>MFKHTRKLQYNAKPDRSDPIMARRLQESLGGQWGETTGMMSYLSQGWASTGAEKYKDLLLDTGTEEMAHVEMISTMIGYLLEDAPFGPEDLKRDPSLATTMAGMDPEHSLVHGLNASLNNPNGAAWNAGYVTSSGNLVADMRFNVVRESEARLQVSRLYSMTEDEGVRDMLKFLLARETQHQLQFMKAQEELEEKYGIIVPGDMKEIEHSEFSHVLMNFSDGDGSKAFEGQVAKDGEKFTYQENPEAMGGI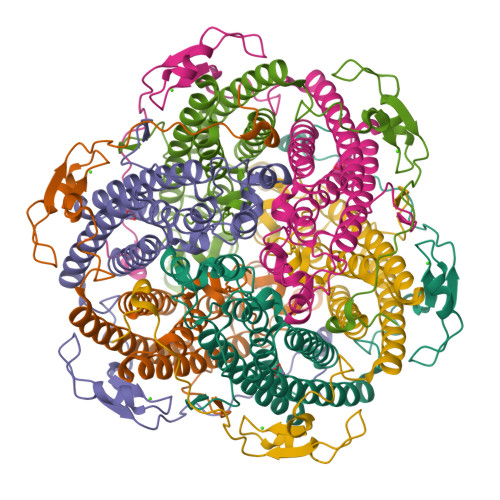PHIKPGDPRLHNHQG[6x]> GSHMTNPQFAGHPFGTTVTAETL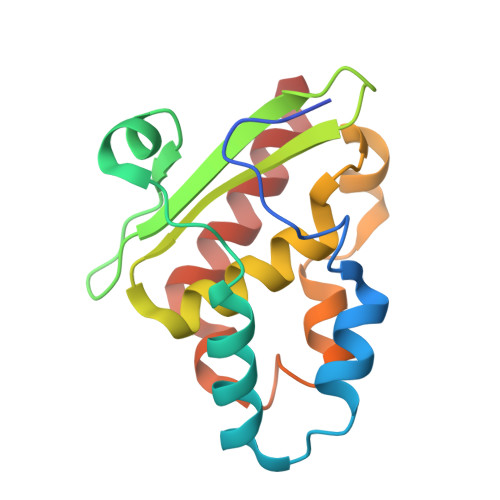RNTFAPLTQWEDKYRQLIMLGKQLPALPDELKAQAKEIAGCENRVWLGYTVAENGKMHFFGDSEGRIVRGLLAVLLTAVEGKTAAELQAQSPLALFDELGLRAQLSASRSQGLNALSEAIIAAAKQV> SNTGNRKYYYIAAEEISWDYSKFVQSDDVDYVPEDTVYKKVVFRKYLDSTFTKLDPQGEYEEHLGILGPVIRAEVDDVIQVRFKNLASRPYSLHAHGLSYEKSSEGKTYEDDSPEWFKEDNAIQPNKTYTYVWHATTRSGPENPGSACRAWAYYSAVNPEKDIHSGLIGPLLICRKGTLDKETNMPVDMREFVLLFMVFDEKKSWYYDKKPTRSWRRASSEVKNSHEFHAINGMIYNLPGLRMYEQEWVRLHLLNLGGSRDIHVVHFHGQTLLENGTQQHQLGVWPLLPGSFKTLEMKASKPGWWLLDTEVGEIQRAGMQTPFLIVDRECKMPMGLSTGLIADSQIQASEFWGYWEPKLARLNNGGSYNAWIAEKLSTEFNPEPWIQVDMQKEVLLTGIQTQGAKHYLKPYYTTEFCVAYSLDRKNWRIFKGNSTRNVMYFGGNSDASTIKENQIDPPVVARYIRISPTGSYNKPALRLELQGCEVNGCSTPLGMESGKIENKQITASSFKKSWWGNYWEPFLARLNAQGRVNAWQAKANNNNQWLQIDLLKIKKITAIVTQGCKSLSSEMYVKSYTIHYSDQGTDWKPYREKSSMVDKIFEGNNNVRGHVKNFFNPPIISRFIRIIPKTWNQ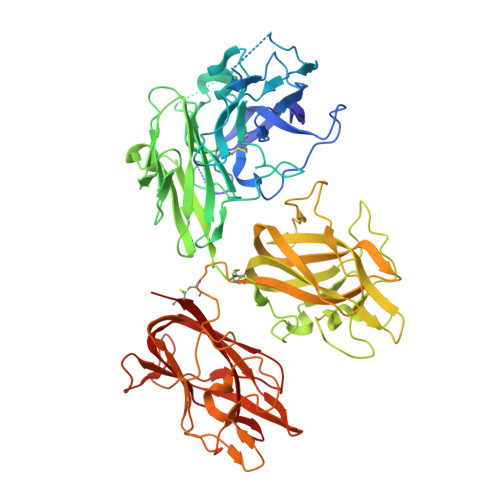SIALRLELFGCDMY Tegumental protein of 20.8 kDa from Clonorchis sinensis elicits IgA immune responses in the host and does not cause an IgG response. For this reason, we named the 20.8-kDa tegumental protein from Clonorchis sinensis as CsTAL3. The interesting thing is that similar results were reported for SmTAL2 and FhCaBP2, 40. Both proteins belong to the TAL protein family of the class of fluke proteins that consist of a calmodulin like domain (or N-terminal domain) and a DLC-like domain (or C-terminal domain) as in CsTAL3. In this work, we determined 2.6 Å crystal structure of the DLC-like domain (amino acid [aa] positions 83–177) and 1.3 Å crystal structure of the calmodulin like domain (aa positions 1–81) of CsTAL3.

At first, we tried crystalizing full-length CsTAL3 (aa 1–184), but the crystal structure contained only the DLC-like domain (aa 83–177). The monomeric structure of the DLC-like domain consists of four anti-parallel β-strands that are packed with each other and an extended loop protruding from β-sheets; the other face of the β-sheets is packed with two α-helices. Despite low sequence identity, the DLC-like domain of CsTAL3 shows structural similarities with the DLC-like domain of FhCaBP2 and 8-kDa human dynein light chain (LC8) with root mean square (r.m.s.) deviation 0.79 and 2.65 Å when 69 Cα and 49 Cα atoms are aligned in Pymol41, respectively. The dimeric interface information calculated by PISA42 is that the dimeric interface area is on average ~1044 Å2 (17.4%) at the total solvent-accessible area of 6033 Å2, and the solvation free energy gain upon formation of the interaction is on average −15.2 kcal/mol. The five residues (G147 to T152) of each protomer in the extended loop interact with five residues (V′142 to D′146) of the neighboring protomer in the β2-strand via a pair of hydrogen bonds. Side chains of these strands also contribute to the hydrophobic interaction. Nonetheless, despite the conservation of the structural characteristics, the amino acid sequences of the dimeric interface are not conserved relative to the other DLC families. The DLC-like domain of CsTAL3 also contains a hydrophobic groove. The superimposition of LC8 with the peptide and DLC-like domain shows a similar conformation. This result suggests that CsTAL3 may interact with its binding partner proteins in a similar manner.

>PSLPPEIIVISANMSLEDQIKIARETIPIAPGAQTSEELGRLTENLKSFADKTFGGCWQVMVVDGSYWITQTFVPNMSFQFELYNRAYLFWQTSE[3x]D,L-endopeptidase RipA is the major PG hydrolase required for daughter cell separation in Mycobacterium tuberculosis ( Mtb ), as RipA defects severely hinder cell division and increase antibiotic vulnerability. Despite extensive studies, the mechanisms governing Mtb RipA regulation remain controversial and poorly understood. Here, we report an integrative structural and functional analysis of the SteAB system, a regulatory complex that has been shown to modulate cell separation in the model organism Corynebacterium glutamicum ( Cglu ) and is conserved across Mycobacteriales .

Although Mtb SteB was previously proposed to act as a mycobacterial outer membrane copper transporter, the crystal structures of the homodimeric protein, alone and in complex with the RipA coiled-coil (CC) domain, rule out this hypothesis. Instead, the high-affinity SteB-RipA interaction, together with computational and biophysical data, strongly supports the role of SteB as a direct RipA activator that releases enzyme autoinhibition upon complex formation. In addition, crystallographic characterization of the cytoplasmic core of SteA revealed a homodimeric organization harboring a conserved functional pocket similar to the phosphonucleotide-binding site of thiamine pyrophosphokinase. These data, coupled with the in vivo phenotypic analysis of a steAB knockout mutant of Cglu , support a model in which the transmembrane SteAB heterotetramer, driven by cytoplasmic ligand binding, orchestrates the productive periplasmic positioning of RipA, leading to PG hydrolysis activation.

> DPQTDTIAALIADVAKANQRLQDLSDEVQAEQESVNKAMVDVETARDNAAAAEDDLEVSQRAVKDANAAIAAAQHRFDTFAAATYMNGPSVSYLSASSPDEIIATVTAAKTLSASSQAVMANLQRARTERVNTESAARLAKQKADKAAADAKASQDAAVAALTETRRKFDEQREEVQRLAAERDAAQARLQAARLVAWSSEGGQGAPPFRMWDPGS;> RSEKRDLYTQIDRLTDQRDALREKLSAADNFDIQVGSRIVHDALVGKSVVIFRTPDAHDDDIAAVSKIVGQAGGAVTATVSLTQEFVEANSAEKLRSVVNSSILPAGSQLSTKLVDQGSQAGDLLGIALLSNADPAAPTVEQAQRDTVLAALRETGFITYQPRDRIGTANATVVVTGGALSTDAGNQGVSVARFAAALAPRGSGTLLAGRDGSANRPAAVAVTRADADMAAEISTVDDIDAEPGRITVILALHDLINGGHVGHYGTGHGAMSVTVSQ>GSAMGSTSRKKVLLKVIILGDSGVGKTSLMNQYVNKKFSNQYKATIGADFLTKEVMVDDRLVTMQIWDTAGLERFQSLGVAFYRGADCCVLVFDVTAPNTFKTLDSWRDEFLIQASPRDPENFPFVVLGNKIDLENRQVATKRAQAWCYSKNNIPYFETSAKEAINVEQAFQTIARNALKQETEVELYNEFPEPIKLDKN[2x];> SAMGNSTGIKLVRKEGGLDDSVFIAVKEIGRDLYRGLPTEERIQK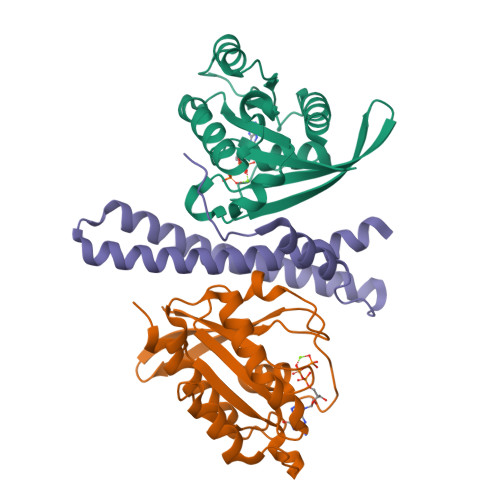LEFMLDKLQNEIDQELEHNNSLVREEKETTDTRKKSLLSAALAKSGERLQALTLLMIHYRAGIEDIETLESLSLDQHSKKISKYTDDT>MKTVHSASYDILRQQGLTTVFGNPGSNELPFLKGFPEDFRYILGLHEGAVVGMADGFALASGQPAFVNLHAAAGTGNGMGALTNAWYSHSPLVITAGQQVRSMIGVEAMLANVDAPQLPKPLVKWSAEPACAEDVPRALSQAIHMANQAPKGPVYLSIPYDDWARPA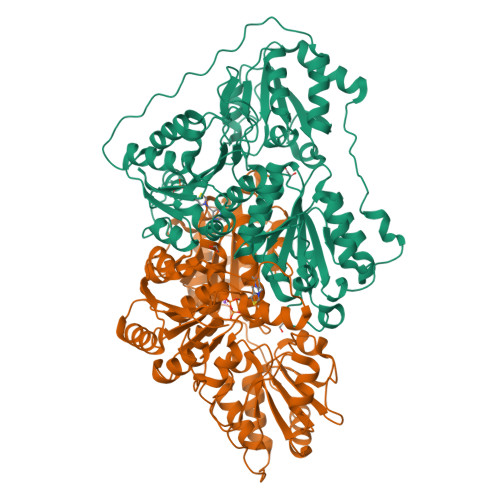PAGVEHLARRQVATAGLPSAAQLRSLVQRLAAARNPVLVLGPDVDGSRSNHLAVQLAEKLRMPAWVAPSASRCPFPTRHPSFRGVLPAAIAGISRCLADHDLILVVGAPVFRYHQFAPGDYLPAGTELLHITCDPGEAARAPMGDALVGDIVETLQALVWALPDCDRPQPQALPPAAPVEELGGLLRPETVFDVIDELAPKDAIYVKESTSTVGAFWQRVEMREPGSYYFPAAGGLGFGLPAAVGVQLARPERRVIGVIGDGSANYGITALWTAAQYQIPVVFIILKNGTYGALRWFAGVLQVSDAPGLDVPGLDFCAIGRGYGVHSVQANTREAFAQALSEALAGDRPVLIEVPTLTIEP[2x]>[2x]GAMDPEFMELRVGNRYRLGRKIGSGSFGDIYLGTDIAAGEEVAIKLECVKTKHPQLHIESKIYKMMQGGVGIPTIRWCGAEGDYNVMVMELLGPSLEDLFNFCSRKFSLKTVLLLADQMISRIEYIHSKNFIHRDVKPDNFLMGLGKKGNLVYIIDFGLAKKYRDARTHQHIPYRENKNLTGTARYASINTH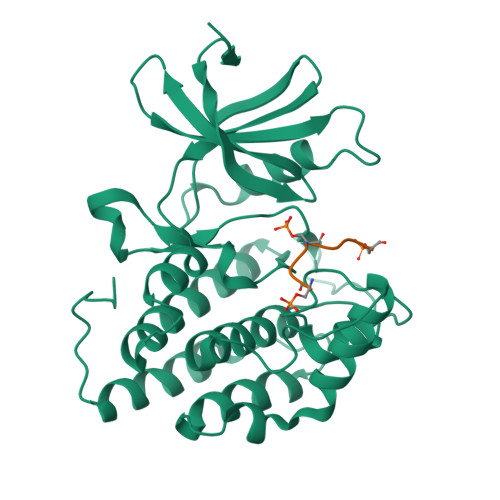LGIEQSRRDDLESLGYVLMYFNLGSLPWQGLKAATKRQKYERISEKKMSTPIEVLCKGYPSEFATYLNFCRSLRFDDKPDYSYLRQLFRNLFHRQGFSYDYVFDWNMLK;>[2x]GKAESVASLTSQ>[4x]MSSELSALVPVLFGHAAFQQLNAGCQLGLFELLHERGPLSAEEVADALRLPRRSADILLLGTTALGLSTVTDGGYRNGAPIGAAFRDGLWPVLRDIVQYQDK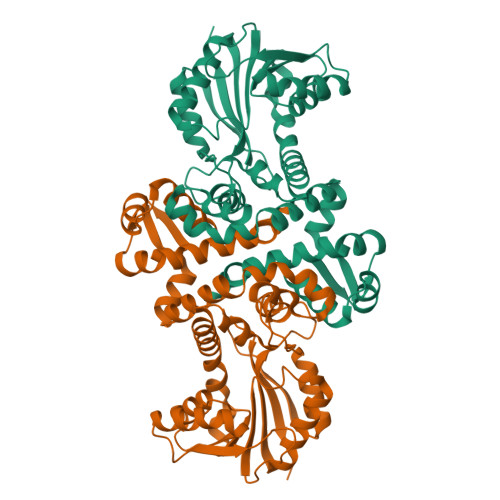IAYQPAADYVESLRTGQNAGIRHFPGTTRDLYSRLAAVPGLEELFYRGMHAWSQLSNPVLLAQPDFTRVHRVLDVGGGDAVNAVALARAHPSLRVTVLDRPGALEVARKTIAEAGLEERVRTHAADIFTDSYPAGHDCVLFAHQLVIWSPEQNLTLLRKAYDAVEPGGRVLVFNAFTDDDRTGPLYAALDNVYFTTLPFRHSTIHRWADCESWLREAGFTDVGRTAPPGWTPHGVVSGSRPRAAALEHHHHHH>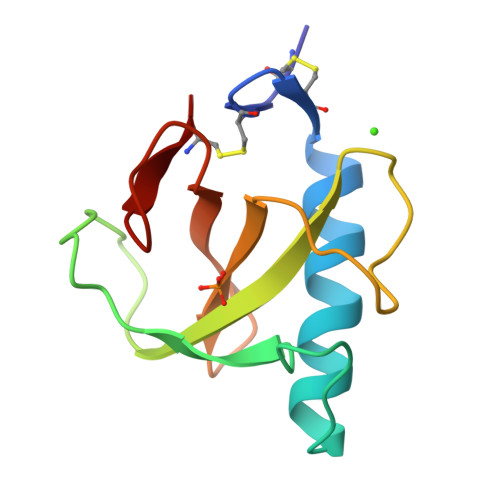 ACDYTCGSNCYSSSDVSTAQAAGYKLHEDGETVGSNSYPKKYNNYEGFDFSVSSPYYEWPILSSGDVYSGGSPGADRVVFNENNQLAGVITHTGASGNNFVECT>[2x]PYVEIIEQPKQRGMRFRYKCEGRSAGS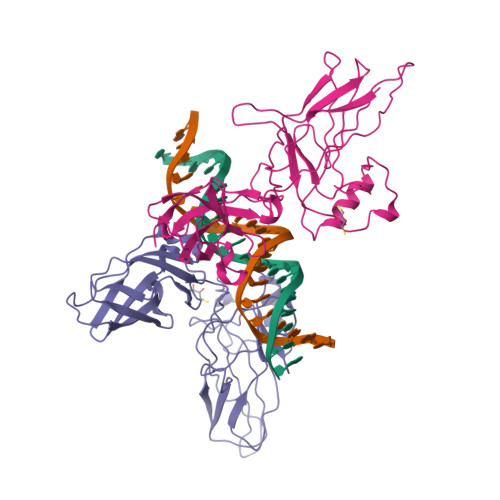IPGERSTDTTKTHPTIKINGYTGPGTVRISLVTKDPPHRPHPHELVGKDCRDGYYEADLCPDRSIHSFQNLGIQCVKKRDLEQAISQRIQTNNNPFHVPIEEQRGDYDLNAVRLCFQVTVRDPAGRPLLLTPVLSHPIFDNRAPNTAELKICRVNRNSGSCLGGDEIFLLCDKVQKEDIEVYFTGPGWEARGSFSQADVHRQVAIVFRTPPYADPSLQAPVRVSMQLRRPSDRELSEPMEFQYLPD>PNNLDSNVSQIVLKKFLPGFMSDLVLAKTVDRQLLAGEINSSTGDSVSFKRPHQFSSLRTPTGDISGQNKNNLISGKATGRVGNYITVAVEYQQLEEAIKLNQLEEILAPVRQRIVTDLETELAHFMMNNGALSLGSPNTPITKWSDVAQTASFLKDLGVNEGENYAVMDPWSAQRLADAQTGLHASDQLVRTAWENAQIPTNFGGIRALMSNGLASRTQGAFGGTLTVKTQPTVTYNAVKDSYQFTVTLTGATASVTGFLKAGDQVKFTNTYWLQQQTKQALYNGATPISFTA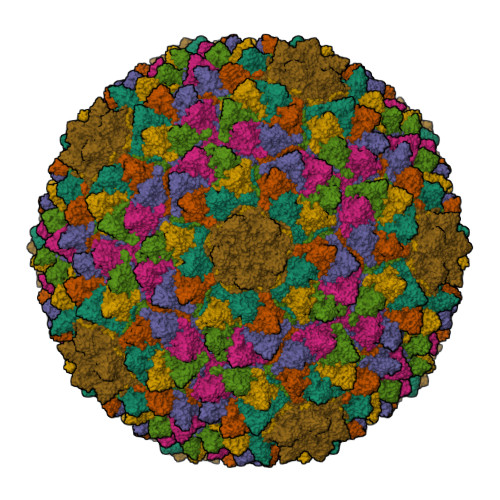TVTADANSDSGGDVTVTLSGVPIYDTTNPQYNSVSRQVEAGDAVSVVGTASQTMKPNLFYNKFFCGLGSIPLPKLHSIDSAVATYEGFSIRVHKYADGDANVQKMRFDLLPAYVCFNPHMGGQFFGNP[7x]>[2x]MVPISPIETVPVKLKPGMDGPKVKQWPLTEEKIKALVEICTEMEKEGKISKIGPENPYNTPVFACKKKDSTKWRKLVDFRELNKRTQDFWEVQLGIPHPAGLKKKKSVTVLDVGDAYFSVPLDEDFRKYTAFTIPSINNETPG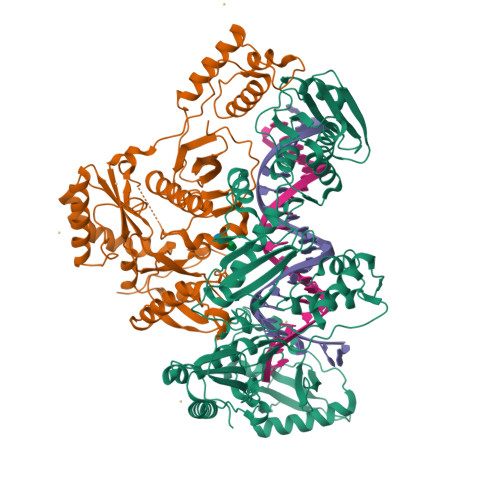IRYQYNVLPQGWKGSPAIFQSSMTKILEPFKKQNPDIVIYQYMDDLYVGSDLEIGQHRTKIEELRQHLLRWGLTTPDKKHQKEPPFLWMGYELHPDKWTVQPIVLPEKDSWTVNDIQKLVGKLNWASQIYPGIKVRQLSKLLRGTKALTEVIPLTEEAELELAENREILKEPVHGVYYDPSKDLIAEIQKQGQGQWTYQIYQEPFKNLKTGKYARMRGAHTNDVKQLTEAVQKITTESIVIWGKTPKFKLPIQKETWETWWTEYWQATWIPEWEFVNTPPLVKLWYQLEKEPIVGAETFYVDGAANRETKLGKAGYVTNKGRQKVVPLTNTTNQKTELQAIYLALQDSGLEVNIVTDSQYALGIIQAQPDKSESELVNQIIEQLIKKEKVYLAWVPAHKGIGGNEQVDKLVSA;>[2x]MAHHHHHHALEVLFQGPISPIETVPVKLKPGMDGPKVKQWPLTEEKIKALVEICTEMEKEGKISKIGPENPYNTPVFAIKKKDSTKWRKLVDFRELNKRTQDFWEVQLGIPHPAGLKKKKSVTVLDVGDAYFSVPLDEDFRKYTAFTIPSINNETPGIRYQYNVLPQGWKGSPAIFQSSMTKILEPFKKQNPDIVIYQYMDDLYVGSDLEIGQHRTKIEELRQHLLRWGLTTPDKKHQKEPPFLWMGYELHPDKWTVQPIVLPEKDSWTVNDIQKLVGKLNWASQIYPGIKVRQLSKLLRGTKALTEVIPLTEEAELELAENREILKEPVHGVYYDPSKDLIAEIQKQGQGQWTYQIYQEPFKNLKTGKYARMRGAHTNDVKQLTEAVQKITTESIVIWGKTPKFKLPIQKETWETWWTEYWQATWIPEWEFVNTPPLVKLWYQ> MVEIAINPASEITATSAFISGTVTKFEQSKGFYGSGCNISLLYWEASNPMHVKVASS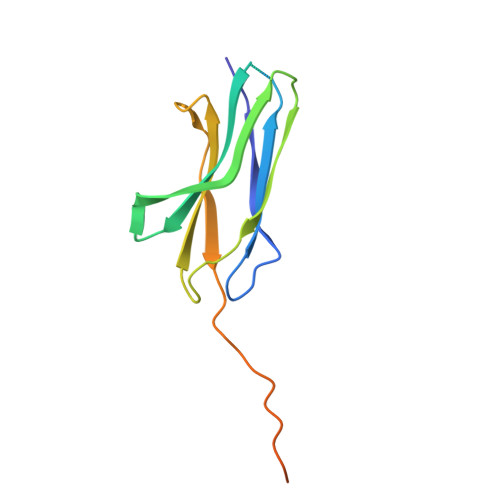ISKKDFPADISATIKDLKPHTTYQFKVTVNFYFSSSLQTFKTLALESKSTSIVSTSTPTPSMPVKVTLEHHHHHH NcCDPK1 is 96% sequence identical to the well-studied TgCDPK1. The structure of NcCDPK1 as seen in both the apo and inhibitor-bound crystals is consistent with the “inactive” forms previously seen in calcium-free crystal structures of CDPK1 homologs from C. parvum (ApiDB_CryptoDB:cgd3_920) and T. gondii (TGME49_101440). In this conformational state the C-terminal Ca2+-binding domain forms a compact structure that occludes the active site of the N-terminal kinase domain, thus preventing the recognition or phosphorylation of substrate proteins.

The observed binding pose of the pyrazolopyrimidine (PP) scaffold and the R1 substituent “bump” in the inhibitor complexes studied here is entirely consistent with that seen previously for PP-scaffold inhibitors bound to the T. gondii homolog. The pose of the piperidine R2 substituent in the current structures is similar but not identical to that seen in TgCDPK1 complexes with other inhibitors containing piperidine ring substituents at this position, which in turn are not identical to each other. This argues for flexibility in the orientation of the piperidine substituents even after binding of these nanomolar inhibitors, and allows additional chemical modifications of this group if necessary to further optimize PK/AMDET properties. The inhibitor structure-activity relationships (SARs) of NcCDPK1 and TgCDPK1 for all compounds tested are virtually identical suggesting that similar BKIs could be useful for both toxoplasmosis and neosporosis therapy. This observation supports our inhibitor-binding mode model derived from BKIs-Tg/NcCDPK1-complex crystal structures that shows favorable interaction of the C3 aryl bump with the gatekeeper hydrophobic pocket. Our data shows 1294 had a 2.6 nM IC50 against NcCDPK1 enzyme and 32 nM EC50 against N. caninum tachyzoites. Compound 1294 was recently shown to be a highly selective inhibitor for parasites' CDPKs compared with 80 mammalian kinases presumably due to smaller gatekeeper residues in CDPKs and other interactions in the CDPKs active sites. Pharmacokinetic data with 1294 demonstrates favorable absorption with low clearance, supporting daily oral administration, and low toxicity in mammalian cells and rodents. We have experimental evidence that N. caninum is prevented from invading the mammalian host cell when lead compound 1294 is added at the time of infection. A therapeutic oral trial with a BKI, 1294, demonstrated marked reduction of N. caninum cerebral parasite burden in mice, thus demonstrating proof-of-concept for neosporosis therapy. The reduced numbers of N. caninum tachyzoites in the brains of treated mice is evidence that compound 1294 crosses the blood-brain barrier in sufficient concentration to be useful in clinical cases.

> GAAGGAGDKLHATPGMFVQHSTAIFSDRYKGQRVLGKGSFGEVILCKDKITGQECAVKVISKRQVKQKTDKESLLREVQLLKQLDHPNIMKLYEFFEDKGYYYLVGEVYTGGELFDEIISRKRFSEVDAARIIRQVLSGITYMHKNKIVHRDLKPENLLLESKSKDANIRIIDFGLSTHFEASKKMKDKIGTAYYIAPEVLHGTYDEKCDVWSTGVILYILLSGCPPFNGANEYDILKKVEKGKYTFELPQWKKVSESAKDLIRKMLTYVPSMRISARDALDHEWIQTYTKEQISVDVPSLDNAILNIRQFQGTQKLAQAALLYMGSKLTSQDETKELTAIFHKMDKNGDGQLDRAELIEGYKELMKMKGQDASMLDASAVEHEVDQVLDAVDFDKNGYIEYSEFVTVAMDRKTLLSRERLERAFRMFDSDNSGKISSSELATIFGVSDVDSETWKNVLAEVDKNNDGEVDFDEFQQMLLKLCGN> AHAAIDTFTKYLDIDEDFATVLVEEGFS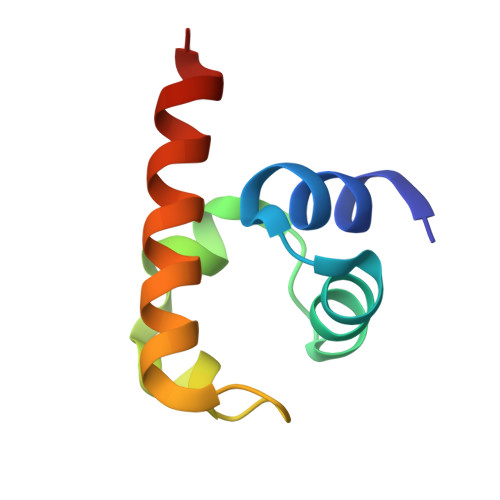TLEELAYVPMKELLEIEGLDEPTVEALRERAKNALATIAQAQ> MSTFGKLFRVTTYGESHCKSVGCIVDGVPPGMSLTEADIQPQLTRRRPGQSKLSTPRDEKDRVEIQSGTEFGKTLGTPIAMMIKNEDQRPHDYSDMDKFPRPSHADFTYSEKYGIKASSGGGRASARETIGRVASGAIAEKFLAQNSNVEIVAFVTQIGEIKMNRDSFDPEFQHLLNT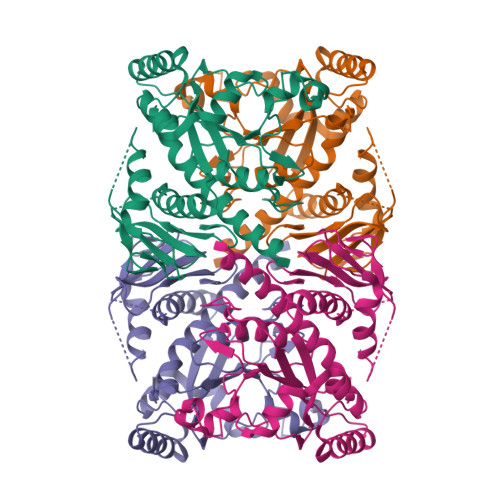ITREKVDSMGPIRCPDASVAGLMVKEIEKYRGNKDSIGGVVTCVVRNLPTGLGEPCFDKLEAMLAHAMLSIPASKGFEIGSGFQGVSVPGSKHNDPFYFEKETNRLRTKTNNSGGVQGGISNGENIYFSVPFKSVATISQEQKTATYDGEEGILAAKGRHDPAVTPRAIPIVEAMTALVLADALLIQKARDFSRSVVHHHHHHH> FM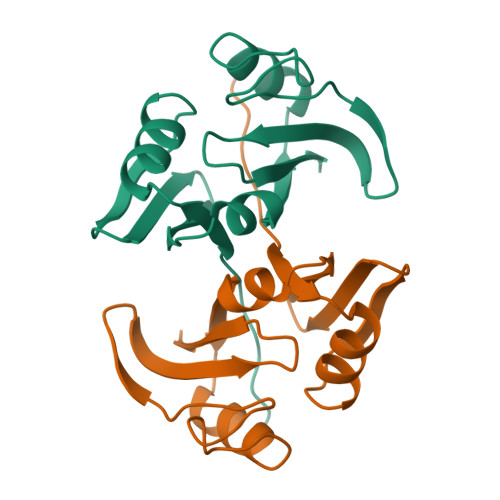AKLTSAVPVLTARDVAGAVEFWTDRLGFSRDFVEDDFAGVVRDDVTLFISAVQDQVVPDNTLAWVWVRGLDELYAEWSEVVSTNFRDASGPAMTEIGEQPWGREFALRDPAGNCVHFVAEEQD>MGFKVKLEKRRNAINTCLCIGLDPDEKDIENFMKNEKENNYNNIKKNLKEKYINNVSIKKDILLKAPDNIIREEKSEEFFYFFNHFCFYIINETNKYALTFKMNFAFYIPYGSVGIDVLKNVFDYLYELNIPTILDMKINDIGNTVKNYRKFIFEYLKSDSCTVNIYMGTNMLKDICYDEEKNKYYSAFVLVKTTNPDSAIFQKNLSLDNKQAYVIMAQEALNMSSYLNLEQNNEFIGFVVGANSYDEMNYIRTYFPNCYILSPGIGAQNGDLHKTLTNGYHKSYEKILINIGRA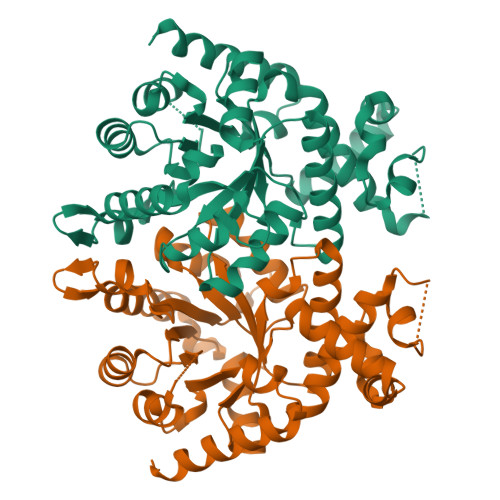ITKNPYPQKAAQMYYDQINAILKQNMES[2x]>[4x]MDIKINDITLGNNSPFVLFGGINVLESLDSTLQTCAHYVEVTRKLGIPYIFKASFDKAARSSIHSYRGVGLEEGLKIFEKVKAEFGIPVITDVHEPHQCQPVAEVCDVIQLPAFLARQTDLVVAMAKTGNVVNIKKPQFLSPSQMKNIVEKFHEAGNGKLILCERGSSFGYDNLVVDMLGFGVMKQTCGNLPVIFDVTHSLQTRDAGSAASGGRRAQALDLALAGMATRLA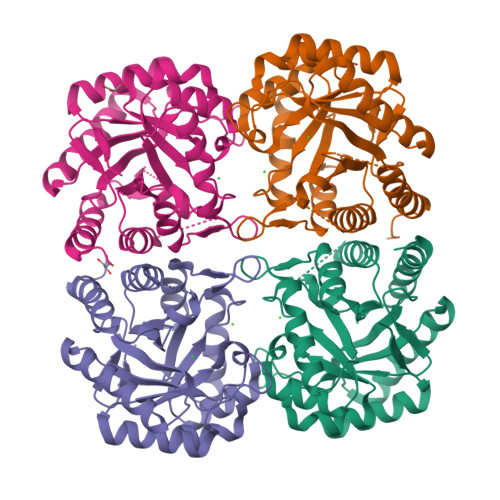GLFLESHPDPKLAKCDGPSALPLHLLEDFLIRIKALDDLIKSQPILTIE>[3x]PAAMF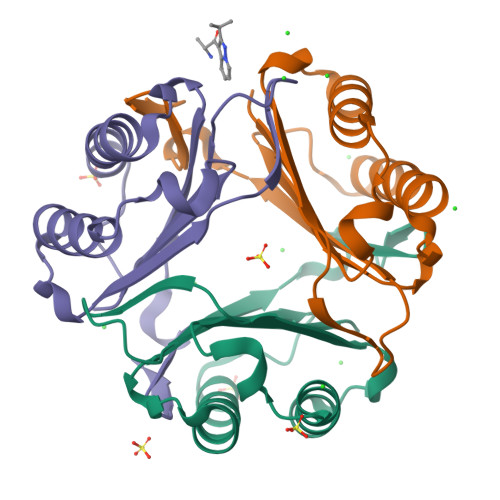IVNTNVPRASVPDGFLSELTQQLAQATGKPPQYIAVHVVPDQLMAFGGSSEPCALCSLHSIGKIGGAQNRSYSKLLCGLLAERLRISPDRVYINYYDMNAANVGWNNSTFA> MLRSTLTSLNTFLTSSVATPPISVIRTGPKWWADPERMVRQKLMYFTLGVDQLP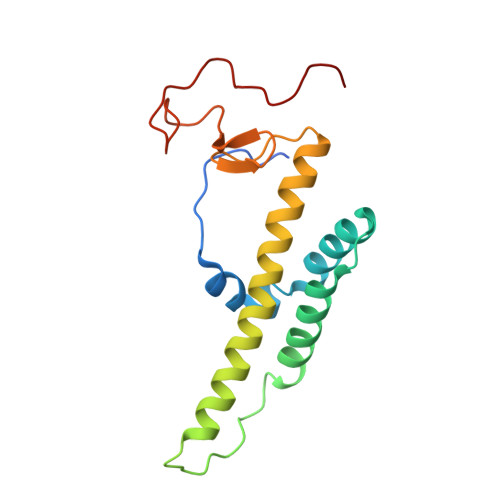LRRTAVIQRDLQRFHMCKPPPRVGDSTGYKRSRAAQLNTWYRRIQYQEYHMQHLFTRHVWGLLRVYPGNTTKIQGKADDGYVGYDSVPFHRYNRAPLPFPARELYERRK>[2x]STAGKVIKCKAAVLWEEKKPFSIEEVEVAPPKAHEVRIKMVATGICRSDDHVVSGTLVTPLPVIAGHEAAGIVESIGEGVTTVRPGDKVIPLFTPQCGKCRVCKHPEGNFCLKNDLSMPRGTMQDGTSRFTCRGKPIH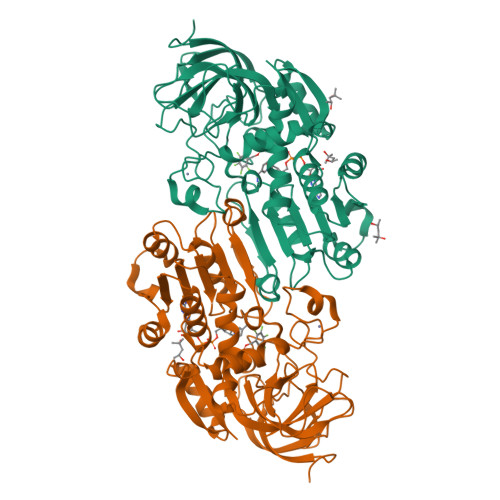HFLGTSTFSQYTVVDEISVAKIDAASPLEKVCLIGCGFSTGYGSAVKVAKVTQGSTCAIFGLGGVGLSVIMGCKAAGAARIIGVDINKDKFAKAKEVGATECVNPQDYKKPIQEVLTEMSNGGVDFSFEVIGRLDTMVTALSCCQEAYGVSVIVGVPPDSQNLSMNPMLLLSGRTWKGAIFGGFKSKDSVPKLVADFMAKKFALDPLITHVLPFEKINEGFDLLRSGESIRTILTF> AAGCUUUUGUGUCUUCAGCUUCCCUCUUCUCCUCGUGGGGUUCCGUUC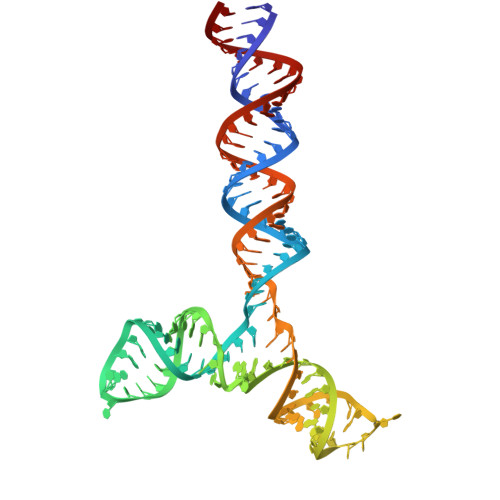CCGCGGUAGUGAGCCUGGUGUGGUUCCGCCCGCGCCAGUGAUGGAGGGUGCUUUAGGCACUAACAAGCUU>GSHMPVVHVIDVESGNLQSLTNAIEHLGYEVQLVKSPKDFNISGTSRLILPGVGNYGHFVDNLFNRGFEKPIREYIESGKPIMGICVGLQALFAGSVESPKSTGLNYIDFKLSRFDDSEKPVPEIGWNSCIPSENLFFGLDPYKRYYFVHSFAAILNSEKKKNLENDGWKIAKAKYGSEEFIAAVNKNNIFATQFHPEKSGKAGLNVIENFLKQQSPPIPNYSAEEKELLMNDYSNYGLTRRIIACLDVRTNDQGDLVVTKGDQYDVREKSDGKGVRNLGKPVQLAQKYYQQGADEVTFLNITSFRDCPLKDTPMLEVLKQAAKTVFVPLTVGGGIKDIVDVDGTKIPALEVASLYFRSGADKVSIGTDAVYAAEKYYELGNRGDGTSPIETISKAYGAQAVVISVDPKRVYVNSQADTKNKVFETEYPGPNGEKYCWYQCTIKGGRESRDLGVWELTRACEALGAGEILLNCIDKDGSNSGYDLELIEHVKDAVKIPVIASSGAGVPEHFEEAFLKTRADACLG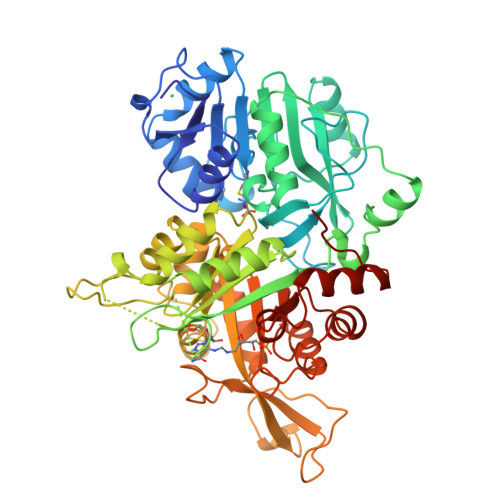AGMFHRGEFTVNDVKEYLLEHGLKVRMDEE[2x]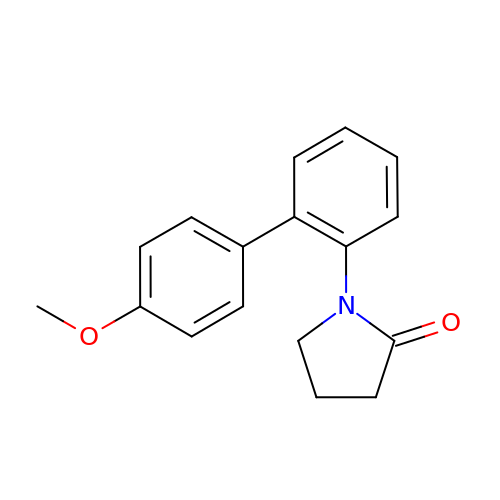1-(4'-methoxy[1,1'-biphenyl]-2-yl)pyrrolidin-2-one | C17 H17 N O2 | GLHCKAVYQJNFHF-UHFFFAOYSA-N> ATTPLCGPSRASIL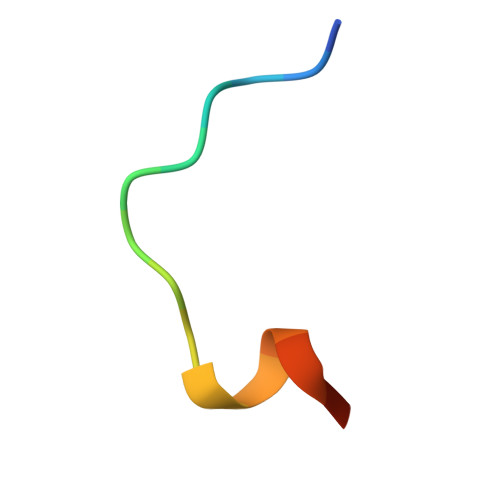SG>[2x]MSVFARLDPELAAALREIPEEFLLDLRDISLARRRLQILREALASLLPPLPSDVAVTDELAPNSFDGTMVRVRLY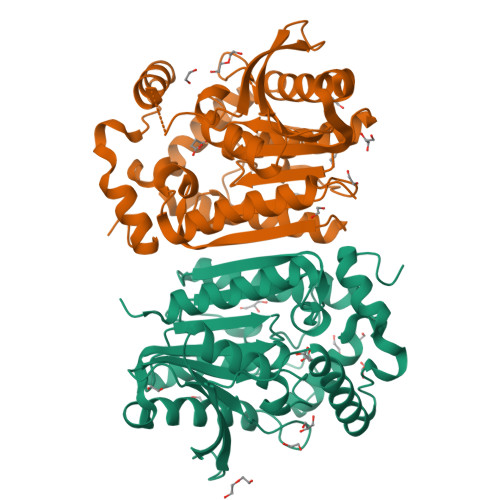RPSEVTGPLPVLLWIHGGGYVMGAPEMNDQQCAELAQRIPALVASVDYRLAPEHPYPAPLEDCYAALRWVAERAEQLGVDRERLAIAGASAGGGLAAGLALLARDRGEVPVRFQLLIYPMLDDRNQTPSSYEITDPRLIWTRDWNLIGWRAYLGREPGSPDVPPYAAPARADDLAGLPPAYVLVGTADLFRDEDIAYAQRLMQAGVPTELHVFAGAFHGFDVFAPTAWVSQRANAEVLAVLQRALKLAAALEHHHHHH>MSTRVYPAQVDVAIVGSGPAGATYARILSERASSATIAMFEVGPTVSDPPGAHVKNIADADERAHAQRRSEGPHAREDDDRVGGIVKSAQRRARPGTYLLESGYQADGEDGLPVAAFSSNVGGMAAHWTGACPRPNDSERIGFLDETGELDELLSEGERLLGVTTDAFDASPYAGIVRERLAAVEDAHRDADERVQRMPLAVHRRDDGPLVWSGSDVVLGDITRGNPNFTLFDESLVTRVLVEDGRAAGVVVTDVRTGERRDVRARFVVVAADALRTPQLLWASGIRPDALGRYLNDQAQIVFAVRMRDFTPV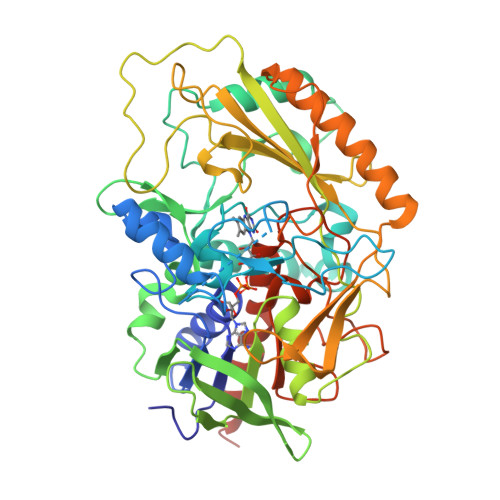VDADGVPQTGLSEYTGVTWVPFTDDMPFHGQVMQLDASPVKLADDDPAAPGSIVGLGLFCAKDLQASDRVAFSDSDVDGYGMPAMQLHYTLSDRDHATIDRAKAEIVRLGKAIGDPLDDRPFVMPLGASLHYQGTVRMGLADDGASVCSPDSEVWGAPGLFVAGNGVIPTATACNPTLTGVALAVRGARHIADEITADLASVKLAAALEHHHHHH[2x]>[4x]ACGLVASNLNLKPGECLRVRGEVAADAKSFLLNLGKDDNNLCLHFNPRFNAHGDVNTIVCNSKDAGAWGAEQRESAFPFQPGSVVEVCISFNQTDLTI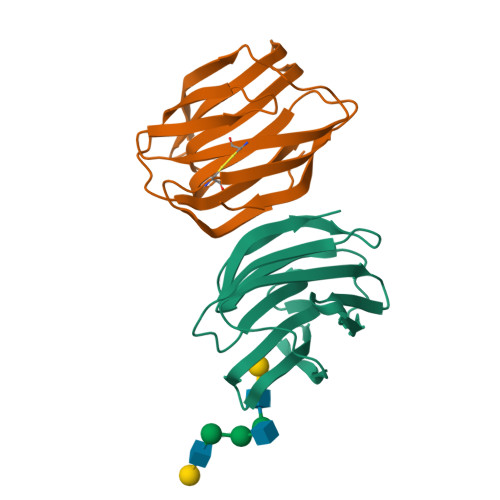KLPDGYEFKFPNRLNLEAINYLSAGGDFKIKCVAFE>GPGSMLACPLPPDEALRQQALDDMALVDTPAEHYLDALVELARETFGVKTVLISLIDHDRQWFKARIGLDAEQTPRDLSFCGHAILASEPLMVTDASRDPRFHDNPLVTGPPFIRFYAGEPLHASNGQAIGTLCLIDPSPRLLDLREGRQLNRLSILAEGYLQLRSLTEHTRFLRQEIDREQRKSLLDPLTQLWNRAGFHALHQHELELARASDQRIGIIYSDIDHFKRINDTLGHRAGDSVLREAASRLRAALRPEDLLARFGGEEFVAMVRVRETTELTMIANRIRELME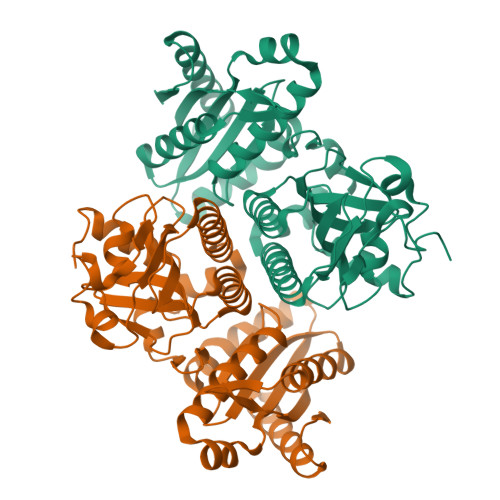ATPIDCAGTSVPVTISAGCTLAGSGEEPERALARADAALYDAKRAGRNRVVSV[4x]>MGRIKNKQFAVIGLGRFGGSICKELHRMGHEVLAVDINEEKVNAYASYATHAVIANATEENELLSLGIRNFEYVIVAIGANIQASTLTTLLLKELDIPNIWVKAQNYYHHKVLEKIGADRIIHPEKDMGVKIAQSLSDENVLNYIDLSDEYSIVELLATRKLDSKSIIDLNVRAKYGCTILAIKHHGDICLSPAPEDIIREQDCLVIMGHKKDIKRFENEGM[2x]

KtrAB is a cation channel with a nucleotide-dependent RCK domain. The structure of the KtrAB complex revealed a homodimeric membrane protein (KtrB) assembled with a cytosolic RCK octameric ring, formed by the KtrA protein. KtrA binds nucleotides, ATP or ADP. ATP binding induces the adoption of a square-conformation by the octameric ring and increased K+ flux activity through KtrAB; ADP binding results in a non-square conformation and decreased flux.

In addition, we crystallized wild-type KtrA-ATP in the presence of 5 mM of Ca2+ and determined the structure at 3.0 Å resolution. The structure shows an octameric ring adopting a square conformation with L1/L2 distances of 30.5/30.5 Å that are similar to those of the WT-ATP structure. The intra-dimer interface shows a bound calcium ion. After refinement, we defined a coordination shell formed by oxygens from the carboxylic groups of the E125 side chains and the oxygen atoms of the ATP γ-phosphates. Unlike what we had observed in the wild-type structure with Mg2+, the R16 side-chains are not in position to coordinate the divalent cation. The coordination distances are consistent with a calcium ion but the coordination number (four ligands) is unusual and there could be additional interactions, with water molecules for example, which we are not currently able to model due to the limited resolution.>[2x]MNTVRSEKDSMGAIDVPADKLWGAQTQRSLEHFRISTEKMPTSLIHALALTKRAAAKVNEDLGLLSEEKASAIRQAADEVLAGQHDDEFPLAIWQTGSGTQSNMNMNEVLANRASELLGGVRGMERKVHPNDDVNKSQSSNDVFPTAMHVAALLALRKQLIPQLKTLTQTLNEKSRAFAD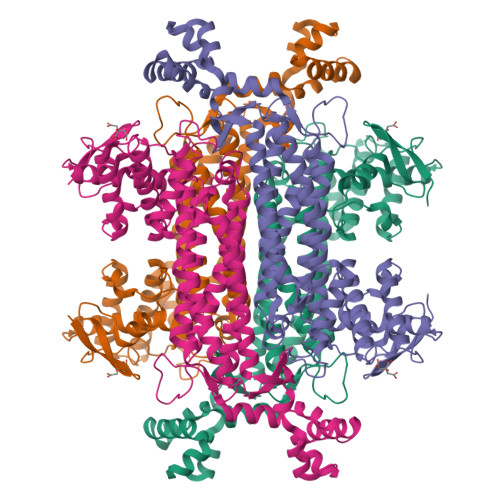IVKIGRTHLQDATPLTLGQEISGWVAMLEHNLKHIEYSLPHVAELALGGTAVGTGLNTHPEYARRVADELAVITCAPFVTAPNKFEALATCDALVQAHGALKGLAASLMKIANDVRWLASGPRCGIGEISIPENEPGSSIMPGKVAPTQCEALTMLCCQVMGNDVAINMGGASGNFELNVFRPMVIHNFLQSVRLLADGMESFNKHCAVGIEPNRERINQLLNESLMLVTALNTHIGYDKAAEIAKKAHKEGLTLKAAALALGYLSEAEFDSWVRPEQMVGSMKAGRHHHHH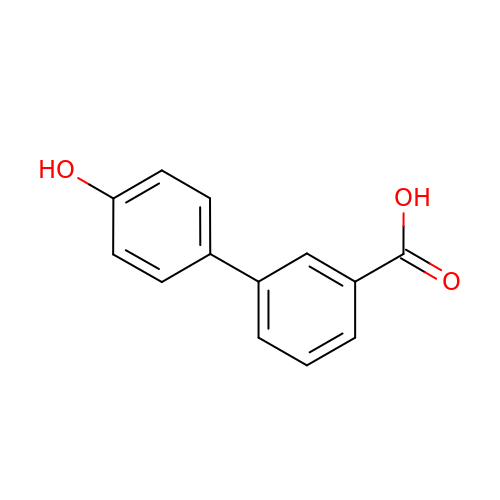3-(4-hydroxyphenyl)benzoic acid | C13 H10 O3 | WINNQOZTIDYENK-UHFFFAOYSA-N>LTAKKRPSVVYLHNAECTGCSESVLRTVDPYVDELILDVISMDYHETLMAGAGHAVEEALHEAIKGDFVCVIEGGIPMGDGGYWGKVGGRNMYDICAEVAPKAKAVIAIGTCATYGGVQAAKPNPTGTVGVNEALGKLGVKAINIAGCPPNPMNFVGTVVHLLTKGMPELDKQGRPVMFFGETVHDNCPRLKHFEAGEFATSFGSPEAKKGYCLYELGCKGPDTYNNCPKQLFNQVNWPVQAGHPCI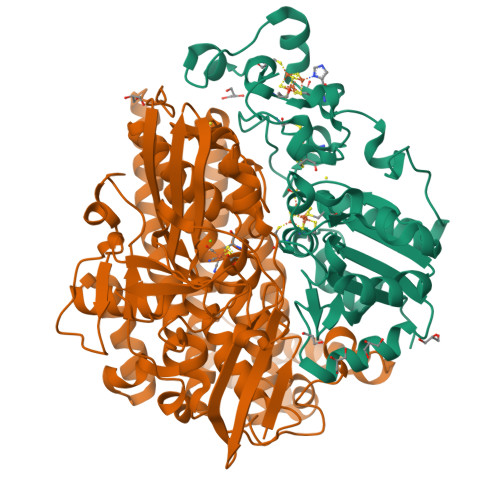ACSEPNFWDLYSPFYSA[2x];>[2x]MSEMQGNKIVVDPITRIEGHLRIEVEVEGGKIKNAWSMSTLFRGLEMILKGRDPRDAQHFTQRACGVCTYVHALASVRAVDNCVGVKIPENATLMRNLTMGAQYMHDHLVHFYHLHALDWVNVANALNADPAKAARLANDLSPRKTTTESLKAVQAKVKALVESGQLGIFTNAYFLGGHPAYVLPAEVDLIATAHYLEALRVQVKAARAMAIFGAKNPHTQFTVVGGCTNYDSLRPERIAEFRKLYKEVREFIEQVYITDLLAVAGFYKNWAGIGKTSNFLTCGEFPTDEYDLNSRYTPQGVIWGNDLSKVDDFNPDLIEEHVKYSWYEGADAHHPYKGVTKPKWTEFHGEDRYSWMKAPRYKGEAFEVGPLASVLVAYAKKHEPTVKAVDLVLKTLGVGPEALFSTLGRTAARGIQCLTAAQEVEVWLDKLEANVKAGKDDLYTDWQYPTESQGVGFVNAPRGMLSHWIVQRGGKIENFQLVVPSTWNLGPRCAEGKLSAVEQALIGTPIADPKRPVEILRTVHSYDPCIACGVH>[4x]MTSASSPPAFRLETSDGDEEGNAEVNKGKQEPPPMESPFQREDRNSSPQIKVNLNFIKRPPKNTSAPSQQEPDRFDRDRLFSVVSRGVPEELTGLLEYLRWNSKYLTDSAYTEGSTGKTCLMKAVLNLQDGVNACIMPLLQIDKDSGNPKLLVNAQCTDEFYQGHSALHIAIEKRSLQCVKLLVENGADVHLRACGRFFQKHQGTCFYFGELPLSLAACTK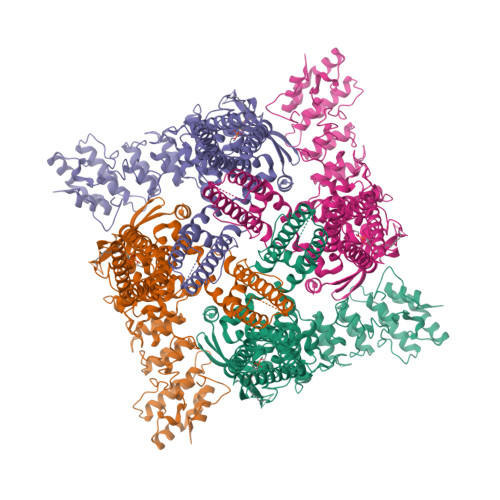QWDVVTYLLENPHQPASLEATDSLGNTVLHALVMIADNSPENSALVIHMYDGLLQMGARLCPTVQLEEISNHQGLTPLKLAAKEGKIEIFRHILQREFSGPYQPLSRKFTEWCYGPVRVSLYDLSSVDSWEKNSVLEIIAFHCKSPNRHRMVVLEPLNKLLQEKWDRLVSRFFFNFACYLVYMFIFTVVAYHQPSLDQPAIPSSKATFGESMLLLGHILILLGGIYLLLGQLWYFWRRRLFIWISFMDSYFEILFLLQALLTVLSQVLRFMETEWYLPLLVLSLVLGWLNLLYYTRGFQHTGIYSVMIQKVILRDLLRFLLVYLVFLFGFAVALVSLSREARSPKAPEDNNSTVTEQPTVGQEEEPAPYRSILDASLELFKFTIGMGELAFQEQLRFRGVVLLLLLAYVLLTYVLLLNMLIALMSETVNHVADNSWSIWKLQKAISVLEMENGYWWCRRKKHREGRLLKVGTRGDGTPDERWCFRVEEVNWAAWEKTLPTLSAAPSGPGITGNKKNPTSKPGKNSASEEDHLPLQVLQSP> SNHTNVKFLFDRSRLLNVIKVLEKDAVFPRPFPTQEGAQQDDGYFCLLTPRPTVASRPATRFGLYANPSGSGVLANTSLDFNFYSLACFTYFRSDLEVTVVSLEPDLEFAVGWFPSGSEYQASSFVYDQLHVPFHFTGRTPRAFASKGGKVSFVLPWNSVSSVLPVRWGGASKLSSATRGLPAHADWGTIYAFVPRPNEKKSTAVKHVAVYIRYKNARAWCPSMLPFRSYK;> GPIPTAPRENSLMFLSTLPDDTVPAYGNVRTPPVNYLPGEITDLLQLARIPTLMAFERVPEPVPASDTYVPYVAVPTQFDDRPLISFPITLSDPVYQNTLVGAISSNFANYRGCIQITLTFCGPMMARGKFLLSYSPPNGTQPQTLSEAMQCTYSIWDIGLNSSWTFVVPYISPSDYRETRAITNSVYSADGWFSLHKLTKITLPPDCPQSPCILFFASAGEDYTLRLPVDCNPSYVF;> RWYTGRLNSWTKAVKTFSFQAVPLPGAFLSRQGGLNGGAFTATLHRHFLMKCGWQVQVQCNLTQFHQGALLVAMVPETTLDVKPDGKAKSLQELNEEQWVEMSDDYRTGKNMPFQSLGTYYRPPNWTWGPNFINPYQVTVFPHQILNARTSTSVDINVPYIGETPTQSSETQNSWTLLVMVLVPLDYKEGATTDPEITFSVRPTSPYFNGLRNRYTAG

Seneca Valley virus (SVV) is an oncolytic picornavirus that selectively targets cancer cells by recognizing Tumor endothelial marker 8 (TEM8) as the host receptor. SVV has a typical picornavirus capsid with four capsid proteins; VP1, VP2, and VP3 are characterized by a single jelly roll fold, where eight beta-strands form a barrel-like structure that is distributed at the exterior of the virus, while VP4 is located on the interior of the capsid. The structural architecture consists of four capsid proteins forming a protomer, 5 protomers forming a pentamer, and 12 pentamers assembling into a pseudo T=3 capsid, approximately ~32 nm in diameter. We used cryo-electron microscopy to investigate SVV under acidic conditions and in complex with TEM8 at physiological pH, identifying multiple uncoating intermediates.

We also imaged SVV complexed with TEM8 under physiological conditions (pH 7 and 37°C). Although the ER-particle from both conditions remains icosahedral, there is a distinct rearrangement of pentamers. Each pentamer has rotated approximately 20° clockwise compared to its position in the F- and A-particles. As a result, the ER-particle is 8% larger than the A-particle and 14% larger than the F-particle, representing a ~44% increase in volume compared to the native state. In the ER-particle[P], these include VP1 (S1-G27), VP2 (D12-D61), and VP4. However, density corresponding to TEM8 becomes visible on the ER-particle when the map is contoured to a low threshold of 0.11. The fact that TEM8 density becomes visible on the ER-particle under physiological conditions potentially suggests that the pentamers or the receptor may adopt a more favorable conformation, enabling a more rigid receptor attachment. The receptor density on the ER-particle[P], although visible only at higher contour levels, supports the idea of functionally significant yet transient receptor interaction during capsid transition. The ER-particle has novel VP2-VP3 and VP3-VP3 contacts at the twofold axis. Overall, the SVV ER-particle is defined by rotated pentamers, an expanded capsid, reduced inter-pentamer contacts, lacks the genome, the VP1 N-terminus, VP2 N-terminus, and the whole of VP4.> IDVSRLDLRIGCIITARKHPDADSLYVEEVDVGEIAPRTVVSGLVNHVPLEQMQNRMVILLCNLKPAK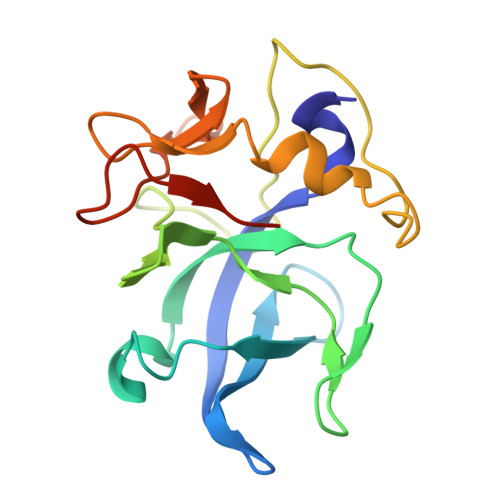MRGVLSQAMVMCASSPEKIEILAPPNGSVPGDRITFDAFPGEPDKELNPKKKIWEQIQPDLHTNDECVATYKGVPFEVKGKGVCRAQTMSNSGIKLEHHHHHH>[24x]SMQRTVARQVALVECVGKGRYGEVWRGLWHGESVAVKIFSSRDEQSWFRETEIYNTVLLRHDNILGFIASDMTSRNSSTQLWLITHYHEHGSLYDFLQRQTLEPHLALRLAVSAACGLAHLHVEIFGTQGKPAIAHRDFKSRNVLVKSNLQCCIADLGLAVMHSQGSDYLDIGNNPRVGTKRYMAPEVLDEQIRTDCFESYKWTDIWAFGLVLWEIARRTIVNGIVEDYRPPFYDVVPNDPSFEDMKKVVCVDQQTPTIPNRLAADPVLSGLAQMMRECWYPNPSARLTALRIKKTLQKISNSPE

Activin receptor-like kinase 1 (ALK1, encoded by the gene ACVRL1) is a type I BMP/TGF-β receptor that mediates signalling in endothelial cells via phosphorylation of SMAD1/5/8. ALK1 synergises with Notch in stalk cells to induce expression of the Notch targets HEY1 and HEY2 and thereby represses tip cell formation and angiogenic sprouting. ALK1 signals via phosphorylation of the transcription factors SMAD1/5/8, which act synergistically with NICD to induce the expression of Notch target genes, including HEY1 and HEY2. Here, we determined the crystal structure of the ALK1 intracellular kinase domain and explored the effects of a small molecule kinase inhibitor K02288 on angiogenesis.

To characterise the homologous structure of human ALK1, we expressed various deletion constructs in Sf9 insect cells and purified the resulting proteins for crystallisation trials. Viable crystals were obtained in the presence of LDN-193189 using a construct comprising ALK1 residues 195–503. The resulting structure was refined at 2.65 Å resolution and defines the kinase domain as well as seven residues from the N-terminal GS domain. Overall, ALK1 adopts an inactive conformation of the kinase domain that is closely conserved with ALK2 (root-mean-square deviation 0.73 Å across 292 Cα atoms). The co-crystallised inhibitor LDN-193189 is bound as expected to the kinase hinge region with a single hydrogen bond to His280. Residues lining the inhibitor binding pocket are strictly conserved between ALK1 and ALK2 explaining their common binding to small molecule BMP inhibitors, including K02288. The ATP pockets of the ALK1 and ALK2 kinase domains are strictly conserved creating a significant challenge for the design of chemical inhibitors that selectively target either protein.>MSQPRTVTVLGATGSIGHSTLDLIERNLDRYQVIALTANRNVKDLADAAKRTNAKRAVIADPSLYNDLKEALAGSSVEAAAGADALVEAAMMGADWTMAAIIGCAGLKATLAAIRKGKTVALANKESLVSAGGLMIDAVREHGTTLLPVDSEHNAIFQCFPHHNRDYVRRIIITASGGPFRTTSLAEMATVTPERAVQHPNWSMGAKISIDSATMMNKGLELIEAFHLFQIPLEKFEILVHPQSVIHSMVEYLDGSILAQIGSPDMRTPIGHTLAWPKRMETPAESLDFTKLRQMDFEAPDYERFPALTLAMESIKSGGARPAVMNAANEIAVAAFLDKKIGFLDI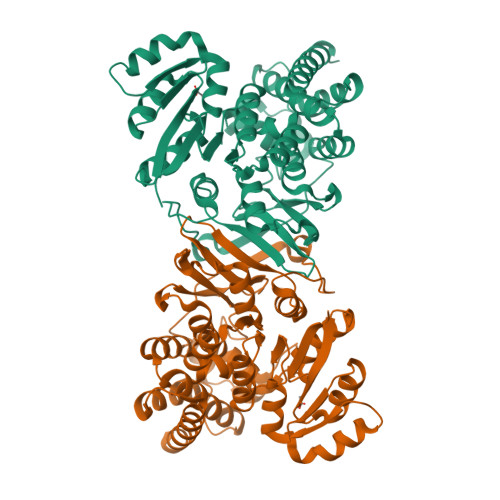AKIVEKTLDHYTPATPSSLEDVFAIDNEARIQAAALMESLPA[4x]>[6x]QSMSLDVHQLSPNEVALMETLLATFGEAFNDMETYTGNRPRG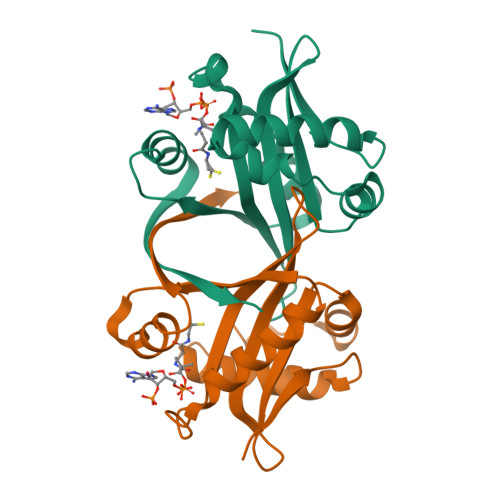AYSRRLLESDYFIALAALEYGEIVGGLAAYELKKFEQERSEIYIYDLAVAKAHRRRGIATALIEKLKELGAARGAYVIFVQADTAIEDEPAIALYSKLGVREEVLHFDIPVSQNNVD> VVGGDECNINEHPFLVALYTSASSTIHCAGALINREWVLTAAHCDRRNIRIKLGMHSKNIRNEDEQIRVPRGKYFCLNTKFPNGLDKDIMLIRLRRPVTYSTHIAPVSLPSRSRGVGSRC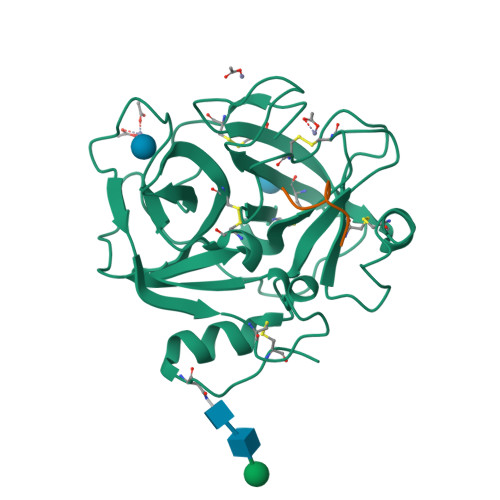RIMGWGKISTTTYPDVPHCTNIFIVKHKWCEPLYPWVPADSRTLCAGILKGGRDTCHGDSGGPLICNGEMHGIVAGGSEPCGQHLKPAVYTKVFDYNNWIQSIIAGNRTVTCPP;> SRDPDNIAAWYLRS> MAASQTSQTVASHVPFADLCSTLERIQKSKGRAEKIRHFREFLDSWRKFHDALHKNHKDVTDSFYPAMRLILPQLERERMAYGIKETMLAKLYIELLNLPRDGKDALKLLNYRTPTGTHGDAGDFAMIAYFVLKPRCLQKGSLTI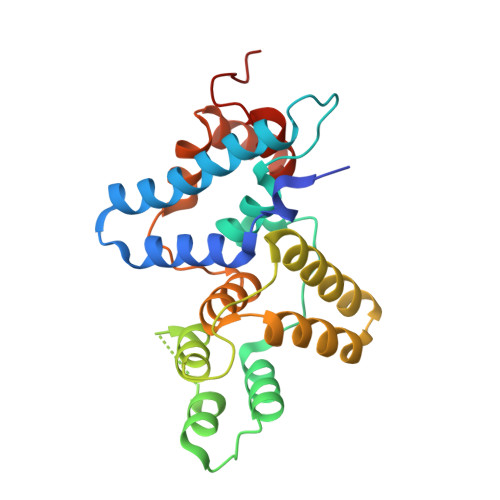QQVNDLLDSIASNNSAKRKDLIKKSLLQLITQSSALEQKWLIRMIIKDLKLGVSQQTIFSVFHNDAAELHNVTTDLEKVCRQLHDPSVGLSDISI UDP-GlcNAc 2-epimerase/ManNAc 6-kinase, GNE, is a bi-functional enzyme that plays a key role in sialic acid biosynthesis. Mutations of the GNE protein cause sialurea or autosomal recessive inclusion body myopathy/Nonaka myopathy. GNE is the only human protein that contains a kinase domain belonging to the ROK (repressor, ORF, kinase) family. Wild type GNE forms homo-hexamer in solution, and allosteric regulation of the epimerase and kinase activities of GNE is important for the normal function of the protein.

Here, we solved the structure of the dimeric GNE kinase domain in the ligand-free state. The overall structure adopts a typical bi-lobal kinase architecture. Residues 475–498 of the N-lobe are invisible in the electron density map. The GNE kinase domain contains a type I zinc-binding motif GHx9–11CxCGx2G(C/H)xE, which forms an HC3 type zinc-finger with residues H569, C579, C581, C586. The kinase domain also contains a DxGxT type ATP-binding motif. Comparison with the actin/hexokinase/hsp70 ATPase domains suggests that the disordered residues 475–498 form part of the binding pocket for the adenosine moiety of ATP and are located near the DxGxT ATP-binding motif. The GNE kinase domain was crystallized in space group P3121 with three molecules in the asymmetric unit. Protein interface and assembly analysis using the PISA server suggests that two of the three molecules dimerize through the C-lobe with an average buried surface area of 1587 Å2 per molecule whereas the third molecule dimerizes with a two-fold symmetry related molecule through the same C-lobe. A crystallographic hexamer can be produced when a two-fold rotational symmetry operation is applied to the three molecules (one and a half dimers) in the asymmetric unit. Two residues, H569 and E588, are located in the ROK family zinc-binding signature motif and H569 directly coordinates the zinc ion.

>MHHHHHHSSGRENLYFQGTLSALAVDLGGTNLRVAIVSMKGEIVKKYTQFNPKTYEERINLILQMCVEAAAEAVKLNCRILGVGISTGGRVNPREGIVLHSTKLIQEWNSVDLRTPLSDTLHLPVWVDNDGNCAALAERKFGQGKGLENFVTLITGTGIGGGIIHQHELIHGSSFCAAELGHLVVSLDGPDCSCGSHGCIEAYASGMALQREAKKLHDEDLLLVEGMSVPKDEAVGALHLIQAAKLGNAKAQSILRTAGTALGLGVVNILHTMNPSLVILSGVLASHYIHIVKDVIRQQALSSVQDVDVVVSDLVDPALLGAASMVLDYTTRR[3x]> MIRAVFFDSLGTLNSVEGHAKMHLKIMEE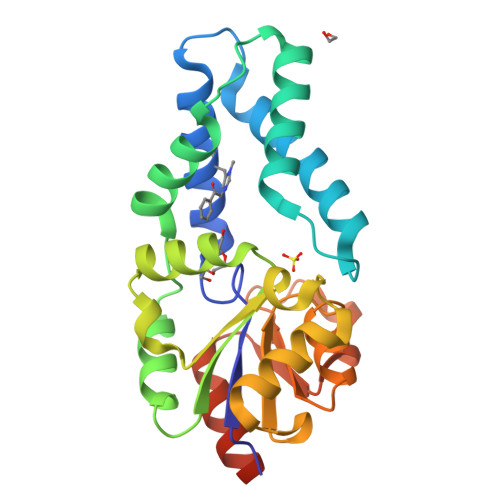VLGDYPLNPKTLLDEYNKLTREAFSNYAGKPYRGLRDILEEVMRKLAEKYGFKYPENFWEISLRMSQRYGELYPEVVEVLKSLKGKYHVGMITDSATEQAMAFLDALGIKDLFDSITTSEEAGFFKPHPRIFELALKKAGVKGEEAVYVGDNPVKDAGGSKNLGMTSILLDRKGEKREFWDKADFIVSDLREVIKIVDELNGQGSLEHHHHHH Here, we present the near-atomic resolution structure of Haloferax tailed virus 1 (HFTV1), an archaeal virus thriving in extreme salinity. Through single-particle analysis, we obtained near-atomic resolution maps of DNA-filled and empty virions, enabling us to assemble full atomic models of the virus pre- and post-DNA release, including all structural protein components. The full atomic structure revealed that the virus has a length of 1350 Å and an icosahedral head with a diameter of ~600 Å. The tail has a length of 560 Å and terminates into a baseplate with three radiating TFs of ~190 Å in length.

The portal is a dodecamer of gp13 (PP), which spans the capsid through one pentagonal vertex. We found that the symmetry mismatch between the MCP pentamer and the PP dodecamer is interfaced by the intermediary portal interface protein gp21 (PIP). A pentameric ring of gp21 (portal interface protein, PIP, brown) integrates the portal 12-mer into the fivefold vertex of the capsid. Around the portal, the conformation of MCP is again different from those found in the trimers, to accommodate the capsid-portal interface. At the portal-capsid interface, one of the MCP-bound magnesium ions is replaced by an arginine of PIP. In addition, PIP also has a putative phosphohistidine residue at position 17, which forms a stabilising H-bond with neighboring MCP monomer. Similarity, but no definite homology, could be determined for the HTC, and the PIP had no hits for structural similarity whatsoever, suggesting that this part of the capsid has a unique origin.

>[30x]MLMEAALPGSDVSAREVAKVWPGAKKGDYSFLQGNQSRSLEAEMTRTARAEAGTDRHRALKDYAVDADNLPKTLSAGSKHLTEDGDVIEARLDDAIPRMLFAASDPEYVDTLFREQLLEVVMEGRELRKVAREASNVINANTRVGDVPIASDEEFARPTGQGAEIRDDGETYTTVAWNATKLTEGSRVTDEMRDQAMVDLIERNIQRVGASLENGINRVFLTELVDNAQNNHDTAGSNQGYQALNSAVGEVDKDDFRPDTYVTHPDYRTQLFNDTNLAYANRAGTNEVLRNREDAPIVGDIAGLDMHAAMSSATYDDGTDIGWSGGSETWGFSSDGDKGAVVYDRDNIHTILYAPNGQDVEIKDYEDPIRDITGVNGRLHVDCQYSQGRSSATVQY;>[15x]MATETQGEHTFPVEVLISGEELRGYTAGEALSAGEPVYLSGDYEVSASSADGGEFLGVNLYDVASGEPVALAGDDCEVRVEVSEQVTANDEILPDGLGTFETVATSAASAGVAIVQEGAASGEVCEAYIFAVQGTTA;>[5x]MQLRRSPGMRPMDRDWHQERARAREQAYSSDLTSQFSESEIVKYELDTAQIDGSDNPRTYIWNRTIDLFGMNGTDVRELRNR;>MPKYNLRIGNRRVPIASTDTPLSEAIGKRLASSTPQTNVDSMGGGHSYQFNGQDLTFEDLRDIKDVRDSGGQVAQLMDYKALLNFGEGCEIHVEGDDETKQLVDGEPMTLSEWLEDAFPHLDLLVLDLGGDALWYPYAVGEIQETITGEFKEALPAEPWTLMPESDAQGKVQAWHQRTKTHGGYQTQTLPADDLWHIVINKASARDEVGISEVLRNKDEIQAFKQNEAAINQAIELHGFPQRHVKVGKEDGAPVRDNDLRRVRTIFDPRTTDANTAYFTGQDVDVETLEAHNFDYSAIHEMDMRNLTTALGLPLEAGNVGADGLGSGKPAELRFALLKLAIKANQRSFSVQFVERVMRPVVRDYSPFDHEADIRLEINDPLEDIGEVADLIQQVGDYMTNEQVAEKLDLPAPEDDEVADSYRSPADMEKDEAGVQDEPFGGMFAGRDMGNRCLGEGITDDELQHAPEWDRPLLEMYQGVTNPESDTSRTLVSFSSSGTPEFVLERIRESIMDGALFSEFDNIPSSRLMELRQTFADELGTDNFTLDSITDALMDFEADLTRDAAERIARTESSAVLNHAREISYEERGEGNELFYWTGADLGDSRQTEACAWLIRQTNPFSGGTPVPMNELRDMVDEAPSHDDSMDNNLARPDSWVVHPNERSSFVKAPPNWEQL[12x];>[12x]MPDPSIDEVSKSDWDALTTQEQDDIISQVENLSSTGWVNTSRERKAEAIRSAIAERDTLYSGNMSRLPTLDGDAEYFTLYLSAHKIQLFEGGEAQSESGEGGSVSYSTGGGGEKDLQKTRYGRMALEYVWEDNSIAALRTY The H. pylori RNA degradosome is composed of RNase J, a 77.6 kDa enzyme that possesses both 5′−3′ exoribonuclease and endoribonuclease activities, and RhpA, a DEAD-box RNA helicase, with a molecular weight of 55.8 kDa2,7. RNase J is essential in H. pylori and plays a major role in the degradation of both mRNAs and antisense RNAs8. The central importance of RNase J in post-transcriptional regulation in H. pylori and its participation in an RNase J-based degradosome prompted us to investigate the structure, oligomeric state and post-translational regulation of the H. pylori RNase J. Here, we report the crystal and cryo-EM structures of H. pylori RNase J that assembles in tetramers organized as a dimer-of-dimers. We also show that in vitro and in solution, RNase J is in equilibrium between dimeric and tetrameric states and our data suggest that the tetrameric form constitutes the active form of RNase J in vitro.

Crystals were prepared from H. pylori RNase J residues 139–691, encompassing the beta-CASP, metallo-beta-lactamase and C-terminal domains. The crystal structure was solved at 2.75 Å by molecular replacement using the Streptomyces coelicolor homolog as a search model. One molecule occupies the asymmetric unit of the crystal, and through crystal symmetry a homotetramer can be generated that is organized as a dimer-of-dimers. The core region of the enzyme, residues 137–586, encompasses the beta-CASP and beta-lactamase domains that define this family, but there are no detectable metal cofactors in the map at the catalytic site. An X-ray fluorescent scan also confirmed that there are no detectable Zn ions in the crystal. The CTD, from residues 587 to 691, is poorly ordered in the crystal lattice and the density was not sufficiently well resolved to model the polypeptide. The structure predicted by the Robetta server is in excellent agreement with the X-ray model for the core, with the notable exception of the three loop regions 174–183, 431–441 and 575–586 at the entrance to the active site, for which the predicted loop positions are closer to those seen in the crystal structure of the S. coelicolor RNase J. The electron density over these regions is well defined in the H. pylori map and modeled with high confidence. An overlay of RNase J of H. pylori and of S. coelicolor, where an RNA substrate is bound, suggests that the path of the RNA to the active site cannot be the same for the two enzymes, and that the nucleic acid would need to be rerouted in the H. pylori enzyme. The obstructions are caused by exposed peptide loop regions that are positioned to accommodate the CTD.

> SKASVKITPLGGLGEIGGNMMVIETPKSAIVIDAGMSFPKEGLFGVDILIPDFSYLHQIKDKIAGIIITHAHEDHIGATPYLFKELQFPLYGTPLSLGLIGSKFDEHGLKKYRSYFKIVEKRCPISVGEFIIEWIHITHSIIDSSALAIQTKAGTIIHTGDFKIDHTPVDNLPTDLYRLAHYGEKGVMLLLSDSTNSHKSGTTPSESTIAPAFDTLFKEAQGRVIMSTFSSNIHRVYQAIQYGIKYNRKIAVIGRSMEKNLDIARELGYIHLPYQSFIEANEVAKYPDNEILIVTTGSQGETMSALYRMATDEHRHISIKPNDLVIISAKAIPGNEASVSAVLNFLIKKEAKVAYQEFDNIHVSGHAAQEEQKLMLRLIKPKFFLPVHGEYNHVARHKQTAISCGVPEKNIYLMEDGDQVEVGPAFIKKVGTIKSGKSYVDNQSNLSIDTSIVQQREEVASAGVFVATIFVNKNKQALLESSQFSSLGLVGFKDEKPLIKEIQGGLEVLLKSSNAEILNNPKKLEDHTRNFIRKALFKKFRKYPAIICHAHSF>[3x]VRNKKVILFDTNHQVSICNQIIDAINSGIDLGDLLEGGLLTLCVEHYYNSDKDKFNTSPIAKYLRDAGYEFDVIKNADATRFLDVIPNEPH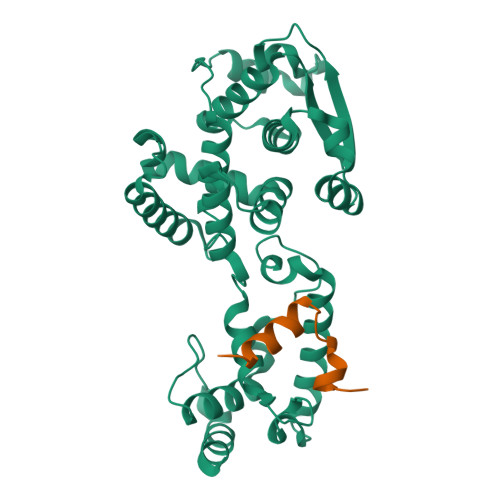YSPLILALKTLESTESQRGRIGLFLSFCSLFLPKLVVGDRASIEKALRQVTVHQEQGIVTYPNHWLTTGHMKVIFGILRSSFILKFVLIHQGVNLVTGHDAYDSIISNSVGQTRFSGLLIVKTVLEFILQKTDSGVTLHPLVRTSKVKNEVASFKQALSNLARHGEYAPFARVLNLSGINNLEHGLYPQLSAIALGVATAHGSTLAGVNVGEQYQQLREAAHDAEVKLQRRHEHQE;>MWDSSYMQQVSEGLMTGKVPIDQVFGAN[3x]>DRHHHHHHKLPEEQKVLVVSFDGFRWDYLYKVPTPHFHYIMKNGVHVNQVTNVFITKTYPNHYTLVTGLFAENHGIVANDMFDPILNKSFSLEHMDIYDSKFWEEATPIWITNQRAGHASGAAM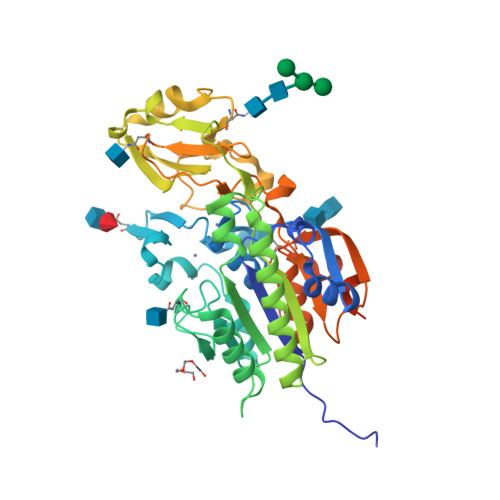WPGADVKIHDSFPTYYLPYNESVSFEDRVAKIIEWFTAKDPINLGFLYWEEPDDTGHDVGPDSPLMGSVISDVDHKLGYLIKMLKRAKLWNNVNLIVTSDHGMTQCSKQRVIELDRYLDKEHYTLIDHSPVAAILPKEGKFDEVYDALAGAHPNLTVYKKEEIPERWHYKHNDRVQPIVAVADEGWYILQNKSDDFLLGNHGYDNALAEMHPIFLAHGPAFRKNFTKEAMNSTDLYSLLCHLLNLTALPHNGSFWNVQDLLSSATPKPIPYTQSTTLLLGSDKPGEDEQEES[2x]>[2x]SNAMSCPVIELTQQLIRRPSLSPDDAGCQALLIERLQAIGFTVERMDFADTQNFWAWRGQGETLAFAGHTDVVPPGDADRWINPPFEPTIRDGMLFGRGAADMKGSLAAMVVAAERFVAQHPNHTGRLAFLITSDEEASAHNGTVKVVEALMARNERLDYCLVGEPSSIEVVGDVVKNGRRGSLTCNLTIHGVQGHVAYPHLADNPVHRAAPFLNELVAIEWDQGNEFFPATSMQIANI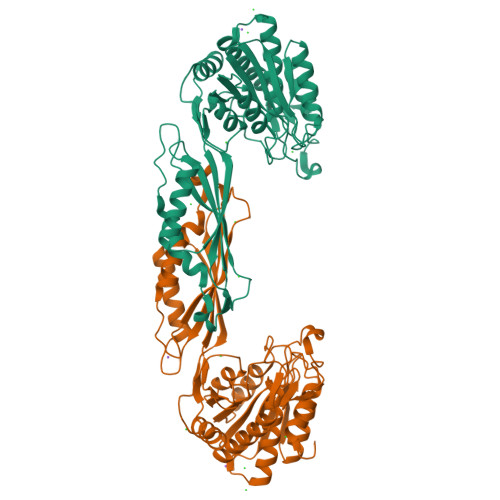QAGTGSNNVIPGELFVQFNFRFSTELTDEMIKAQVLALLEKHQLRYTVDWWLSGQPFLTARGKLVDAVVNAVEHYNEIKPQLLTTGGTSDGRFIARMGAQVVELGPVNATIHKINECVNAADLQLLARMYQRIMEQLVA> MLDPNLLRTEPDAVAEKLARRGFKLDVDKLRALEERRKVLQVQTENLQAERNSRSKSIGQAKARGEDIEPLRLEVNKLGEQLDAAKSELETLLAEIRDIALAIPNIPHDDVPVGRDENDNVEVSRWGTPRQFDFEVRDHVTLGEMHGGLDFAAAVKLTGSRFVVMKGQLARLHRALAQFMLDLHTEQHGYSENYVPYLVNQDTLYGTGQLPKFAGDLFHTRPLEEEADSSNYALIPTAEVPLTNLVRDEIIDEDDLPIKMTAHTPCFRSEAGSYGRDTRGLIRMHQFDKVEMVQIVRPEDSMAALEEMTGHAEKVLQLLGLPYRKVALCTGDMGFSACKTYDLEVWVPAQNTYREISSCSNVWDFQARRMQARCRSKSDKKTRLVHTLNGSGLAVGRTLVALMENYQQADGRIEIPEVLRPYMRGLEYIG

The aminoacyl-tRNA synthetases (aaRSs) are essential enzymes playing a central role in the translation of the genetic code and hence constitute a viable target for the development of antibiotics. Based on the structure of the catalytic site, two distinct classes of tRNA synthetases can be discerned. Both classes activate an amino acid in forming the respective aminoacyl-adenylate (aa-AMP) as natural reaction intermediates. In view of their resemblance and irrespective of the class, aminoacyl-sulfamoyl adenosine (aaSA) derivatives are well-known high-affinity aaRS inhibitors, but they lack antibacterial activity due to their low uptake potential. Structural analysis showed the flipped 2-hydroxymethyl-1,3-dideazaadenine base is partially mimicking the interactions of adenine within both series of aaRS enzymes.

For class II aaRSs, the adenine makes numerous interactions with active site residues, with the N1, N3 and N6 all making H-bond interactions with conserved features shared amongst all class II aaRS members. The interaction between the N3 of adenine with the conserved water molecule for class II aaRS enzymes is crucial for the recognition of aaSAs by the corresponding enzymes. It was hypothesized that the flipped exocyclic amine moiety of HMDDA should be able to mimic this specific interaction. However, in the case of SerRS, the base moiety adopts the syn-conformation relative to the ribose defined by the torsion angle (O4′-C1′-N7-C8) of −124°, while the base bound in the active site of class I LeuRS and TyrRS and class II AspRS remains in the anti-conformation. In this specific syn conformation in SerRS, the hydroxymethyl group of the base forms a direct H-bond with the carbonyl oxygen of Met284, and N9 makes an indirect contact with the backbone nitrogen of Met284 via a water bridge. Despite the HMDDA base making some interactions with surrounding protein residues, compared with the adenine congener, the lack of H-bonds mediated by N6 and N3 of adenine with the conserved Glu270 and structural water molecule leads to a detrimental effect on its inhibitory activity. However, in class II aaRSs, two different base conformations were observed, where the base adopts an anti-conformation in AspRS as seen in class I aaRSs but a syn conformation in SerRS. This is likely the result of the distinct flexibility of their motif-2 loop regions. A comparison of ligand-free and ligand-bound states shows that the motif-2 loop is in a relative fixed position (a closed conformation) in SerRS independently of inhibitors binding, while this loop region in AspRS is more dynamic, which has been described in detail in our previous work. While these values reflect high affinity for the target enzymes, the inhibition is 5 to 420-fold lower compared to that with the original aaSA analogue.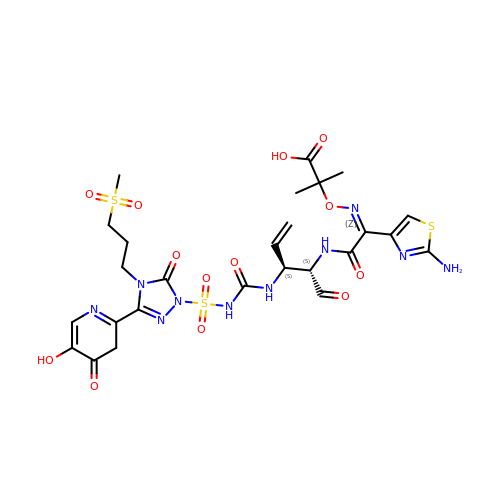(3S,4S,7Z)-7-(2-amino-1,3-thiazol-4-yl)-3-ethenyl-4-formyl-1-[({3-(5-hydroxy-4-oxo-3,4-dihydropyridin-2-yl)-4-[3-(methylsulfonyl)propyl]-5-oxo-4,5-dihydro-1H-1,2,4-triazol-1-yl}sulfonyl)amino]-10,10-dimethyl-1,6-dioxo-9-oxa-2,5,8-triazaundec-7-en-11-oic acid | C26 H32 N10 O13 S3 | AHKKXUZADGDRIH-JNUWSLPISA-N> GPDEEPEEPGRRGSFVEMVDNLRGKSGQGYYVEMTVGSPPQTLNILVDTGSSNFAVGAAPHPFLHRYYQRQLSSTYRDLRKGVYVPYTQGKWEGELGTDLVSIPHGPNVTVRANIAAITESDKFFINGSNWEGILGLAYAEIARPDDSLEPFFDSLVKQTHVPNLFSLQLCGAGFPLNQSEVLASVGGSMIIGGIDHSLYTGSLWYTPIRREWYYEVIIVRVEINGQDLKMDCKEYNYDKSIVDSGTTNLRLPKKVFEAAVKSIKAASSTEKFPDGFWLGEQLVCWQAGTTPWNIFPVISLYLMGEVTNQSFRITILPQQYLRPVEDVATSQDDCYKFAISQSSTGTVMGAVIMEGFYVVFDRARKRIGFAVSACHVHDEFRTAAVEGPFVTLDMEDCGYNI

BACE‐1 is a membrane‐bound aspartyl protease required for the processing of the amyloid precursor protein (APP) to form the N‐terminus of Aβ peptides and the protein‐soluble APPβ (sAPPβ) (Vassar et al, 1999). The beta‐site amyloid precursor protein cleaving enzyme‐1 (BACE‐1) initiates the generation of amyloid‐β (Aβ), and the amyloid cascade leading to amyloid plaque deposition, neurodegeneration, and dementia in Alzheimer's disease (AD). Subsequent intramembrane proteolysis catalyzed by the γ‐secretase complex releases amyloid‐β peptides of 38–43 amino acids, which form the pathogenic oligomeric and fibrillary Aβ species. Inhibition of BACE‐1 by low‐molecular‐weight compounds has emerged as a new concept for treatment of AD (Vassar et al, 2014; Eketjall et al, 2016; Kennedy et al, 2016; Timmers et al, 2016, 2017; Yan et al, 2016; Cebers et al, 2017) by preventing the generation and deposition of Aβ rather than just treating the dementia symptoms.

We present here the structure of the BACE‐1 inhibitor CNP520 for the first time. It is the result of extensive structural optimization of the 3‐amino‐1,4‐oxazine lead series of BACE‐1 inhibitors and a detailed understanding of CNP520's binding to BACE‐1. B X‐ray structure of CNP520 bound to the BACE‐1 active site (resolution: 1.35 Å), with binding pockets S1 (filled by P1) and S3 (filled by P3) and catalytic residues Asp32 and Asp228. The amino‐oxazine head group mediates the key binding interactions to Asp32 and Asp228 in BACE‐1, but, being the most polar part of the molecule, it also largely determines the permeation and distribution properties of CNP520. Consequently, the basicity of the cyclic amidine of CNP520 was fine‐tuned to pKa = 7.2 by introduction of the electron‐withdrawing trifluoromethyl group. Furthermore, we speculated that a bulky group at position 2 of the oxazine ring might reduce binding of CNP520 to P‐gp, a major drug transporter located at the blood–brain barrier responsible for drug efflux. BACE‐1 shares high structural similarity with the catalytic and ligand binding sites of these enzymes; however, we increased selectivity for BACE‐1 by exploiting the size differences of remote substrate binding pockets, in particular the extended S3 pocket. We discovered that a picolinic acid with para‐trifluoromethyl substitution, pointing into the extended S3 pocket, provided threefold selectivity for BACE‐1 over BACE‐2 and 20,000‐fold selectivity for BACE‐1 over CatD, which translated to functional selectivity in vivo (see below). Finally, we identified the central fluoropyridyl moiety as a non‐genotoxic building block that could replace earlier aniline‐type substructures that generated aniline metabolites upon hydrolysis of the amide bond (Neumann et al, 2015). Enzyme inhibition assays showed CNP520 to be a potent BACE‐1 inhibitor that is selective for BACE‐1 over other human pepsin‐like aspartic proteases, including BACE‐2 and CatD.>[2x]MGSLEKFNLIDEPWIPVLKGGRVVEVGIGEALLRAHEFARIETPSPLEEAVLHRLLLAVLHRALSGPRCPEDVLDWWRKGGFPQDPIRDYLNRFRDRFFLFHPEAPFLQVADLPEENPLPWSKLLPELASGNNPTLFDHTTEENLPKATYAQAARALLVHQAFAPGGLLRRYGVGSAKDAPVARPALFLPTGQNL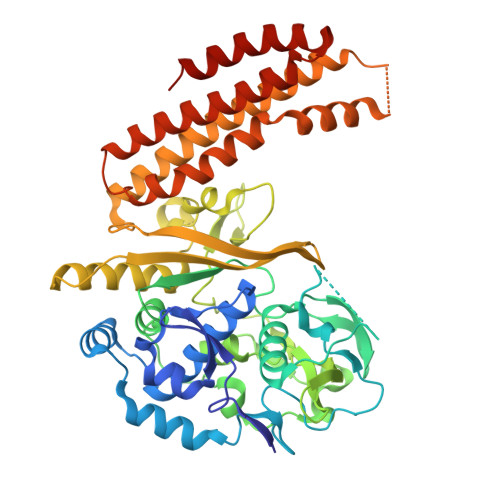LETLLLNLVPYTPEDDAPIWEVPPLRLGDLEGARTKWPLTGRTRVYTWPARGVRLLDEGDGVRFMGYGPGVEPLEATHRDPMVAQRLDAKGNLLVLRLSEERSFWRDFSAMLPRQGGKVAATLEHAENLQGELEDEGLEGRITLRVLGQVSDQAKVLDIRREVYPLPSGLLTPKAEENLEKALKMAEELGQGLKHLAQEVAKAVVGERDRGHGRSPYLEELTKLANSLPLERLYWHALDGAFPRFFARVEEEASLDLWREALRGAALEAWKATRRFLGTGARHLKALAQGEQEFGRLLGELGEEVRT>GGVEVLEVKTGVDAITEVECFLNPEMGDPDENLRGFSLNLSAENDFSSDSPQRKMLPCYSTARIPLPNLNEDLTSGNLLMWEAVTVQTEVIGITSMLNLHAGSQKVHEHGGGKPIQGSNF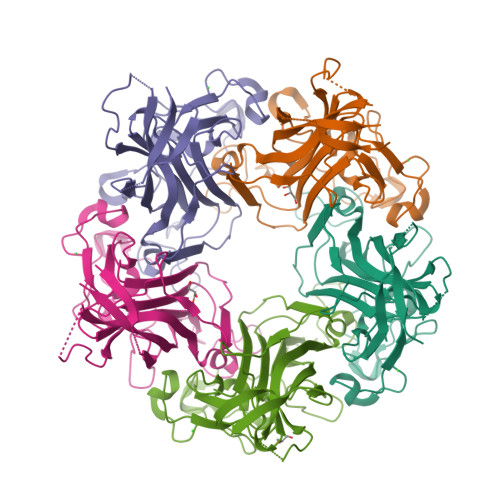HFFAVGGEPLEMQGVLMNYRSKYPDGTITPKNPTAQSQVMNTDHKAYLDKNNAYPVECWVPDPSRNENARYFGTFTGGENVPPVLHVTNTATTVLLDEQGVGPLCKADSLYVSAADICGLFTNSSGTQQWRGLARYFKIRLRKRSVKNPYP[10x]> NQSVVVDFLLPTGVYLNFPVSRNANLSTIKQLLWHRAQYEPLFHMLSGPEAYVFTCINQTAEQQELEDEQRRLCDVQPFLPVLRLVAREGDRVKKLINSQISLLIGKGLHEFDSLCDPEVNDFRAKMCQFCEEAAARRQQLGWEAWLQYSFPLQLEPSAQTWGPGTLRLPNRALLVNVKFEGSEESFTFQVSTKDVPLALMACALRKKATVFRQPLVEQPEDYTLQVNGRHEYLYGSYPLCQFQYICSCLHSGLTPHLTMVHSSSILAMRDEQSNPAPQVQKPRAKPPPIPAKKPSSVSLWSLEQPFRIELIQGSKVNADERMKLVVQAGLFHGNEMLCKTVSSSEVSVCSEPVWKQRLEFDINICDLPRMARLCFALYAVIEKAKKARSTKKKSKKADCPIAWANLMLFDYKDQLKTGERCLYMWPSVPDEKGELLNPTGTVRSNPNTDSAAALLICLPEVAPHPVYYPALEKILELGRHSECVHVTEEEQLQLREILERRGSGELYEHEKDLVWKLRHEVQEHFPEALARLLLVTKWNKHEDVAQMLYLLCSWPELPVLSALELLDFSFPDCHVGSFAIKSLRKLTDDELFQYLLQLVQVLKYESYLDCELTKFLLDRALANRKIGHFLFWHLRSEMHVPSVALRFGLILEAYCRGSTHHMKVLMKQGEALSKLKALNDFVKLSSQKTPKPQTKELMHLCMRQEAYLEALSHLQSPLDPSTLLAEVCVEQCTFMDSKMKPLWIMYSNEEAGSGGSVGIIFKNGDDLRQDMLTLQMIQLMDVLWKQEGLDLRMTPYGCLPTGDRTGLIEVVLRSDTIANIQLNKSNMAATAAFNKDALLNWLKSKNPGEALDRAIEEFTLSCAGYCVATYVLGIGDRHSDNIMIRESGQLFHIDFGHFLGNFKTKFGINRERVPFILTYDFVHVIQQGKTNNSEKFERFRGYCERAYTILRRHGLLFLHLFALMRAAGLPELSCSKDIQYL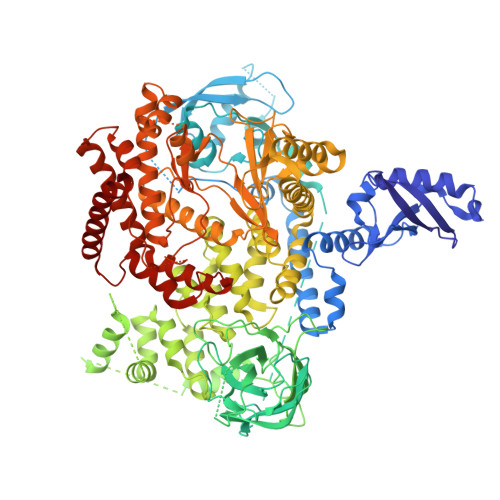KDSLALGKTEEEALKHFRVKFNEALRESWKTKV[(1E)-1-nitroprop-1-en-2-yl]benzene | C9 H9 N O2 | 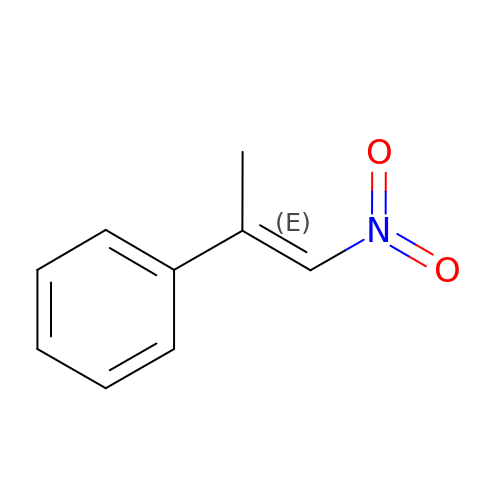KFNFMBKUWFTFAE-BQYQJAHWSA-N>[2x]HHHHHHENLYFQGMTVQKTVDSRIPTLIRNGLQTKKRSFFVVVGDHAKEAIVHLYYIMSSMDVRQNKSVLWAYKKELLGFTSHRKKREAKIKKEIKRGIREPNQADPFELFISLNDIRYCYYKETDKILGNTYGMCILQDFEAITPNILARTIETVEGGGLVVLLLKGMTSLKQLYTMTMDVHARYRTEAHDDVIARFNERFLLSLGSCESCLVIDDELNVLPISGGKGVKPLPPPDEDEELSPAAKELKKIKDELEDTQPIGSLIKLARTVDQAKALLTFVDAIAEKTLRNTVTLTAARGRGKSAAMGVAIAAAVAYGYSNIFITSPSPENLKTLFEFVFKGFDALDYKDHADYTIIQSTNPEFNKAIVRVNIHRNHRQTIQYIRPQDAHVLGQAELVVIDEAAAIPLPLVKKLMGPYLVFMASTISGYEGTGRSLSLKLIKQLREQSRAGANPNGG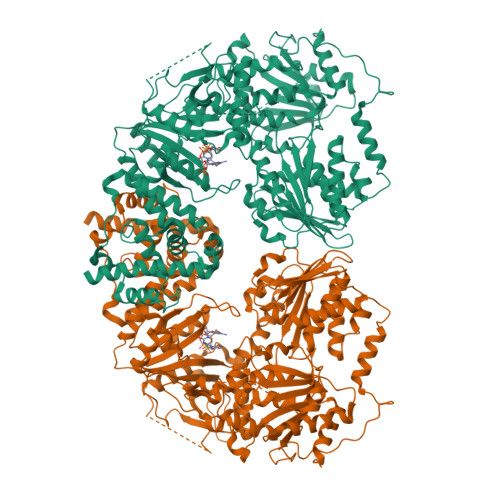NAVEVDRSTLKATKETTSVGGRSLKEITLSEPIRYAQGDNVEKWLNTLLCLDATLPRSKISTTGCPDPSQCELLHVNRDTLFSFHPVSEKFLQQMVALYVASHYKNSPNDLQLMSDAPAHELFVLTGPIQEGRLPEPLCVIQVSLEGKISKQSILKSLSRGQQPAGDLIPWLVSQQFQDDEFASLSGARIVRIATNPDYMSMGYGSKALQLLVDYYEGKFADLSEDAAAEVPRSIPRVTDAELSKGSLFDDIKVRDMHELPPLFSKLSERRPEKLDYVGVSYGLTQQLHKFWKRAQFVPVYLRQTANDLTGEHTCVMIRPLQDGNDPSWLGAFAADFHKRFLSLLSYKFREFPSILALTIEESANAGAMLDPSNAPTELTKAELDQLFTPFDHKRLESYANGLLDYHVVLDLMPTIAQLYFTGRLREAVKLSGLQQAILLALGLQRKDIDTLATELNLPGSQVLAIFMKIMRKVTQHFGALVSGAIAAELPDPNKTVGVSKENAMGIHDDEVVGLKFEALEQRLEDELDEGGDEALRELRKKQRELIDSLPLDQYEIDGDDDAWKEAEKRVASAAKSGKKVDGTLVSVPSAKAAKRKAEEMAALRDELEKMEKGKERGSKKAKKEKRR>MERYRRGMEILNRMNRKSYTAIRDELEDVAPDLARFVAEFAYGDVYSRGVLD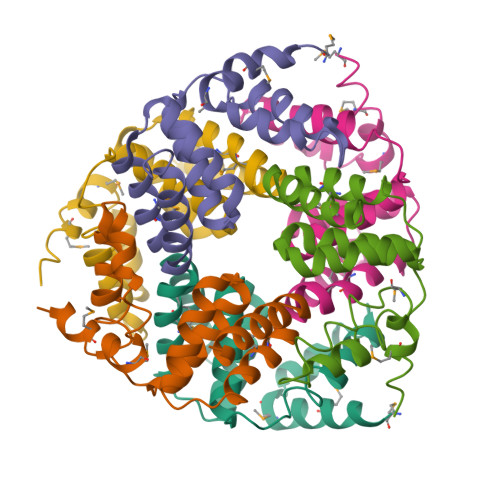LKTRELLTLAALTVLRADDQLKSHVRGALNAGCSKDEIIEVMIQMAVYAGFPAAINAVLAAKEVFTENDPAEV[9x]> GMPDIFQQEARGWLRCGAPPFAGAVAGLTTKHGGESKGPFASLNMGLHVGDDRTDVVNNRRRLAEWLAFPLERWVCCEQVHGADIQKVTKSDRGNGAQDFATAVPGVDGLYTDEAGVLLALCFADCVPIYFVAPSAGLVGLAHAGWRGTAGGIAGHMVWLWQTREHIAPSDIYVAI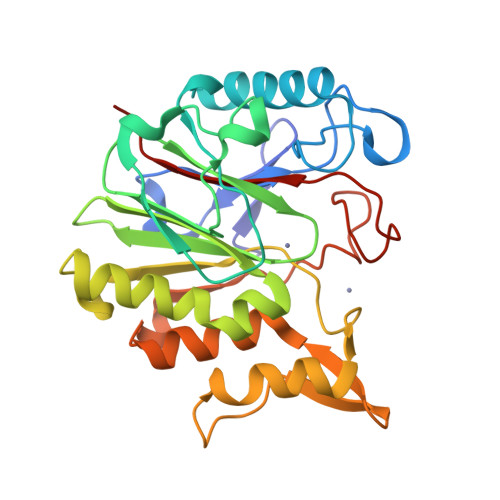GPAIGPCCYTVDDRVVDSLRPTLPPESPLPWRETSPGQYALDLKEANRLQLLAAGVPNSHIYVSERCTSCEEALFFSHRRDRGTTGRMLAFIGRREEWT> MSIDTARSGSDDDVEIREIQAAAAPTRFARGWHCLGLLRDFQDGKPHSIEAFGTKLVVFADSKGQLNVLDAYCRHMGGDLSRGEVKGDSIACPFHDWRWNGKGKCTDIPYARRVPPIAKTRAWTTLERNGQLYVWNDPQGNPPPEDVTIPEIAGYGTDEWTDWSWKSLRIKGSHCREIVDNVVDMAHFFYIHYSFPRYFKNVFEGHTATQYMHSTGREDVISGTNYDDPNAELRSEATYFGPSYMIDWLESDANGQTIETILINCHYPVSNNEFVLQYGAIVKKLPGVSDEIAAGMAEQFAEGVQLGFEQDVEIWKNKAPIDNPLLSEEDGPVYQLRRWYQQFYVDVEDITEDMTKRFEFEIDTTRAVASWQKEVAENLAKQAEGSTATP;> MSLGTSEQSEIREIVAGSAPARFARGWHCLGLAKDFKDGKPHSVHAFGTKLVVWADSNDEIRILDAYCRHMGGDLSQGTVKGDEIACPFHDWRWGGNGRCKNIPYARRVPPIAKTRAWHTLDQDGLLFVWHDPQGNPPPADVTIPRIAGATSDE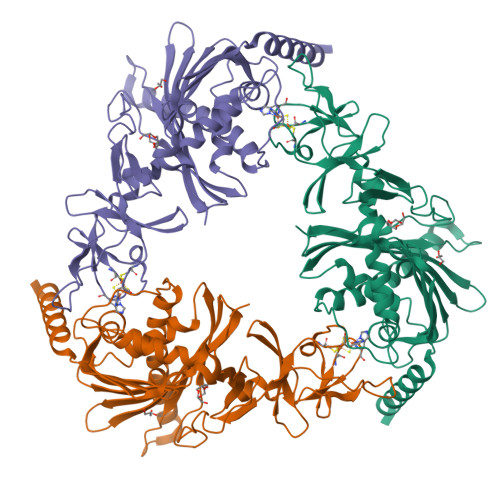WTDWVWYTTEVDTNCREIIDNIVDMAHFFYVHYSFPVYFKNVFEGHVASQFMRGQAREDTRPHANGQPKMIGSRSDASYFGPSFMIDDLVYEYEGYDVESVLINCHYPVSQDKFVLMYGMIVKKSDRLEGEKALQTAQQFGNFIAKGFEQDIEIWRNKTRIDNPLLCEEDGPVYQLRRWYEQFYVDVEDVAPEMTDRFEFEMDTTRPVAAWMKEVEANIARKAALDTETRSAPEQSTTAG> SSL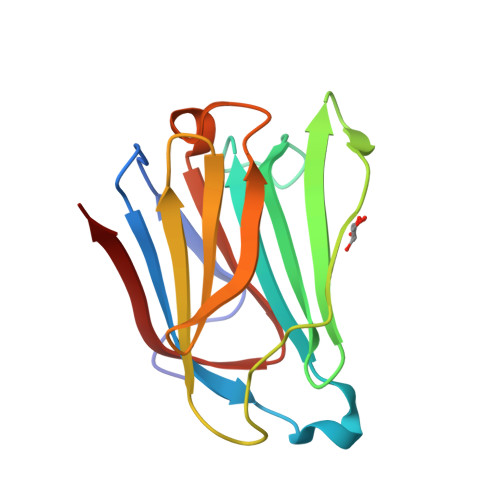PVPYKLPVSLSVGSCVIIKGTPIHSFINDPQLQVDFYTDMDEDSDIAFHFRVHFGNHVVMNRREFGIWMLEETTDYVPFEDGKQFELCIYVHYNEYEIKVNGIRIYGFVHRIPPSFVKMVQVSRDISLTSVCVCN> SGVDDDMAC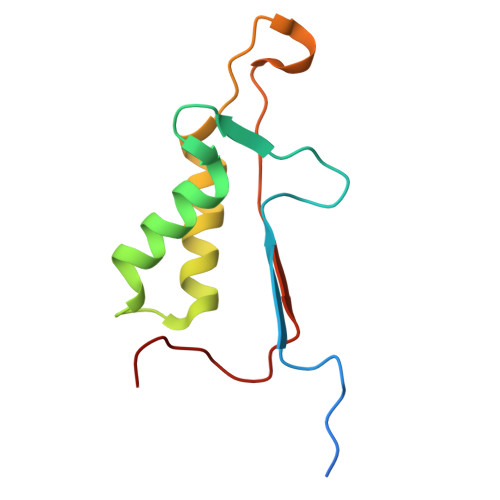HKIPVEADFLYAYSTAPGYYSWRNSKDGSWFIQSLCAMLKQYADKLEFMHILTRVNRKVADEFESFSFDATFHAKKQIPCIVSMLTKELYFYH> SSNSEFDDATTEFETPELFKPSLCYKFNDGSSYTITNQDFKCLFNKDWVNDSILDFFTKFYIESSIEKSIIKREQVHLMSSFFYTKLISNPADYYSNVKKWVNNTDLFSKKYVVIPINISYHWFSCIITNLDAILDFHQNKDKNDAINSDEISINNPLVNILTFDSLRQTHSREIDPIKEFLISYALDKYSIQLDKTQIKMKTCPVPQQPNMSDCGVHVILNIRKFFENPVETIDVWKNSKI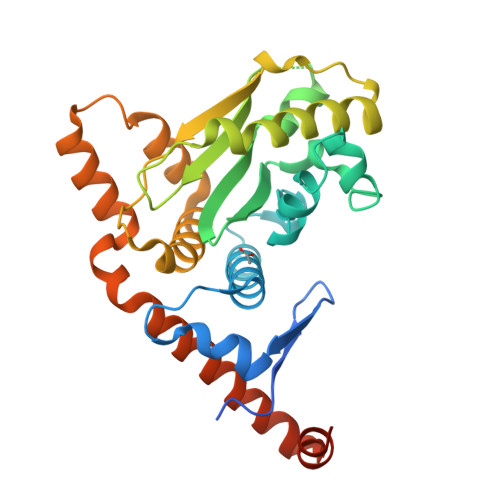KSKHFTAKMINKYFDKNERNSARKNLRHTLKLLQLNYISYLKKENLYEEVMQMEEKKSTGGGHHHHHH>GLEDCDFGWSPYDQHCYQAFNEQKTWDEAEKFCRAQENGAHLASIESNGEADFVSWLISQKDELADEDYVWIGLRAQNKEQQCSSEWSDGSSVSYENLIDLHTKKCGALEKLTGFRKWVNYYCEQMHAFVCKLLPY[2x];>[2x]MGRFIFVSFGLLVVFLSLSGTGADCPSGWSSYEGHCYKPFNEPKNWADAERFCKLQPKHSHLVSFQSAEEADFVVKLTRPRLKANLVWMGLSN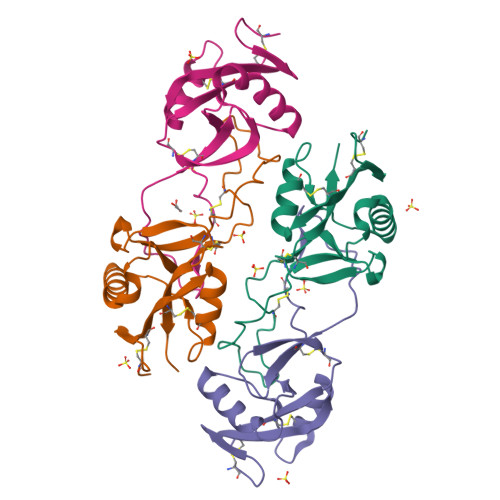IWHGCNWQWSDGARLNYKDWQEQSECLAFRGVHTEWLNMDCSSTCSFVCKFKA> TAATTSQPAFSPDQVSVIFVLGGPGAGKGTQCEKLVKDYSFVHLSAGDLLRAEQGRAGSQYGELIKNCIKEGQIVPQEITLALLRNAISDNVKANKHKFLIDGFPRKMDQAISFERDIVESKFILFFDCPEDIMLERLLERGKTSGRSDDNIESIKKRFNTFKETSMPVIEYFETKSKVVR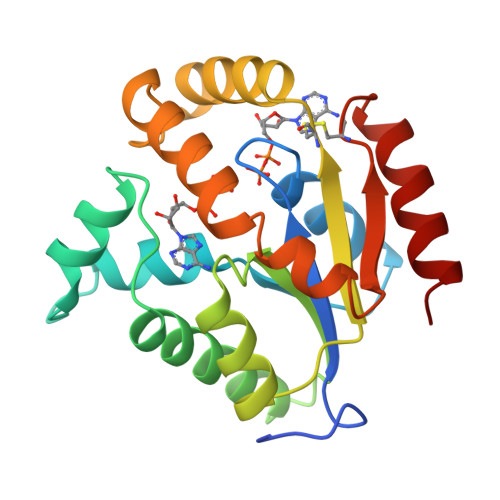VRCDRSVEDVYKDVQDAIRDSL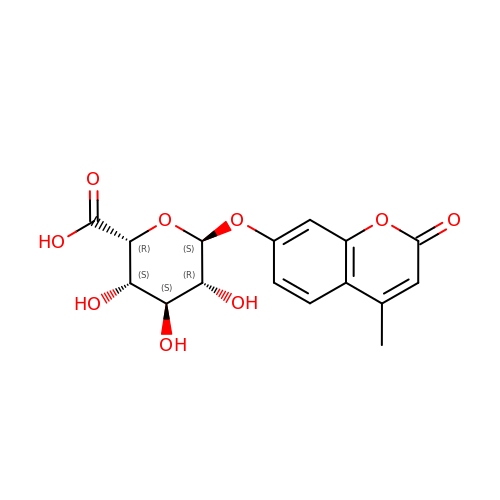(2~{R},3~{S},4~{S},5~{R},6~{S})-6-(4-methyl-2-oxidanylidene-chromen-7-yl)oxy-3,4,5-tris(oxidanyl)oxane-2-carboxylic acid | C16 H16 O9 | ARQXEQLMMNGFDU-ZHMBSYLPSA-N> MMENKTETTVRRRRRIILFPVPFQGHINPILQLANVLYSKGFSITIFHTNFNKPKTSNYPHFTFRFILDNDPQDERISNLPTHGPLAGMRIPIINEHGADELRRELELLMLASEEDEEVSCLITDALWYFAQSVADSLNLRRLVLMTSSLFNFHAHVSLPQFDELGYLDPDDKTRLEEQASGFPMLKVKDIKSAYSNWQILKEILGKMIKQTKASSGVIWNSFKELEESELETVIREIPAPSFLIPLPKHLTASSSSLLDHDRTVFQWLDQQPPSSVLYVSFGSTSEVDEKDFLEIARGLVDSKQSFLWVVRPGFVKGSTWVEPLPDGFLGERGRIVKWVPQQEVLAHGAIGAFWTHSGWNSTLESVCEGVPMIFSDFGLDQPLNARYMSDVLKVGVYLENGWERGEIANAIRRVMVDEEGEYIRQNARVLKQK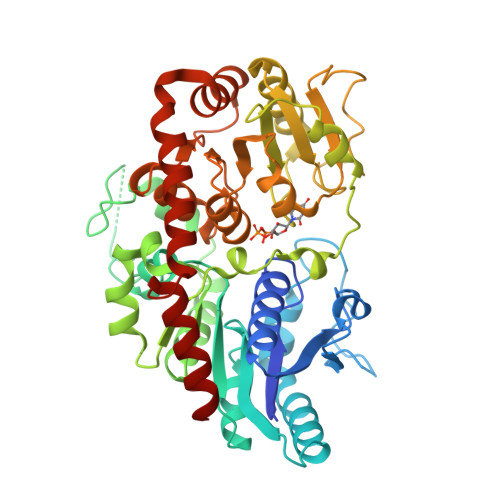ADVSLMKGGSSYESLESLVSYISSLTS>LSSSPSEILQELGKGSTHPQPGVSPPAAPAAPGPKDGPGETDAFGNSEGKELVASGENKIKQGLLPSLEDLLFYTIAEGQEKIPVHKFITALKSTGLRTSDPRLKECMDMLRLTLQTTSDGVMLDKDLFKKCVQSNIVLLTQAFRRKFVIPDFMSFTSHIDELYESAKKQSGGKVADYIPQLAKFSPDLWGVSVCTADGQRHSTGDTKVPFCLQSCVKPLKYAIAVNDLGTEYVHRYVGKEPSGLRFNKLFLNEDDKPHNPMVNAGAIVVTSLIKQGVNNAEKFDYVMQFLNKMAGNEYVGFSNATFQSERESGDRNF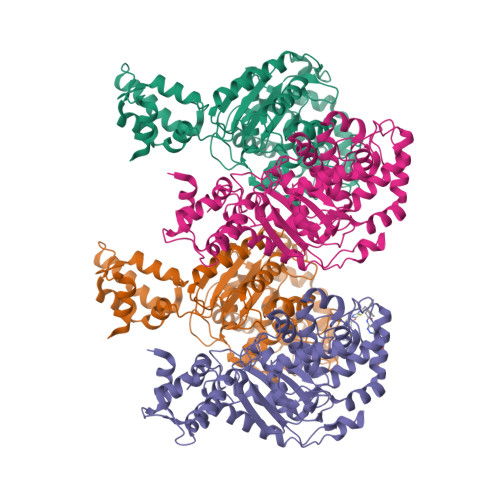AIGYYLKEKKCFPEGTDMVGILDFYFQLCSIEVTCESASVMAATLANGGFCPITGERVLSPEAVRNTLSLMHSCGMYDFSGQFAFHVGLPAKSGVAGGILLVVPNVMGMMCWSPPLDKMGNSVKGIHFCHDLVSLCNFHNYDNLRHFAKKLDPRREGGDQRHSFGPLDYESLQQELALKETVWKKVSPESNEDISTTVVYRMESLGEKS[4x]> GSSPVQSGFNNGTISNYMYFERRPDLLTKGTQDKAAAVKLKIENFYQSSVKYAIERNERRVELETELTSHNWSEERKSRQLSSLGKKESQFLRLRRTRLSLEDFHTVKVIGKGAFGEVRLVQKKDTGKIYAMKTLLKSEMYKKDQLAHVKAERDVLAGSDSPWVVSLYYSFQDAQYLYLIMEFLPGGDLMTMLIRWQL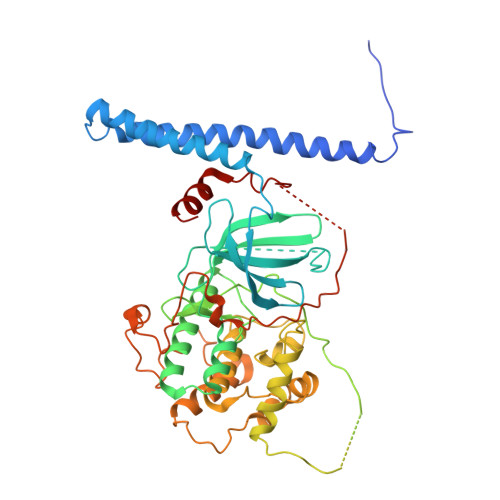FTEDVTRFYMAECILAIETIHKLGFIHRAIKPDNILIDIRGHIKLSDFGLSTGFHKTHDSNYYKKLLQQDEATNGISKPGTYNANTTDTANKRQTMVVDSISLTMSNRQQIQTWRKSRRLMAYSTVGTPDYIAPEIFLYQGYGQECDWWSLGAIMYECLIGWPPFCSETPQETYRKIMNFEQTLQFPDDIHISYEAEDLIRRLLTHADQRLGRHGGADEIKSHPFFRGVDWNTIRQVEAPYIPKLSSITDTRFFPTDELENVPDSPAMAQAAKQREQMTKQGGSAPVKEDLPFIGYTYSRFDYLTRKNAL>MKKLVMTAAVAAILGAASPVMAQGIPVFDGTRALDFVQQFARMKEQLDTAKDQLAEAQRMYEAVTGGRGLGDLMRNAQLREYLPDDLRTVYDSANGGGYSGISGSINDILRDERLNGSVADMRRSIEERSRTAAATDKAVGLRAYEGAQQRLAQIEGLMDEISRTQDQKAIEELQARIAGEQAAIQNETTKLQMIAQLRQAEQALISEQRRERNMRILSSGNQGMPTIQ[5x];>MSKKQPKPVKAEQLKSYYEESRGLERDLIGEFVKSRKTAWRVATASGLFGLLGMVCGIVGFSQPAPAPLVLRVDNATGAVDVVTTLREHESSYGEVVDTYWLNQYVLNREAYDYNTIQMNYDTTALLSAPAVQQDYYKLFDGSNARDRVLGNKARITVRVRSIQPNGRGQATVRFTTQQHNSNGTVEAPQHQIATIGYTYIGAPMRSSDRLLNPLGFQVTSYRADPEILNN[12x];>[5x]MAFELFTPLFNKIDQTTATYVTDISSRAIAAITPVVSVGLTLGFITYGWLIIRGAVEMPVAEFLNRCLRIGIIVSIALAGGLYQGEIANAITTVPDELASALLGNPTQGASAAALVDQSAQQGFDRASEAFEEAGFFSSDGLLYGLFGIIILLATGLLAAIGGAFLLLAKIALALLAGLGPLFILALIWQPTHRFFDQWAQQVLNYGLLIVLFAAVFGLLMQIFGSYMADLRFDGAQNVAYAIGGSVILSIVSIVLLMQLPSIASGLAGGIGLGYMWELRSMRSGAGAAMRGGRAMARGARAAPGAARGAAVGAANMAKTVATGGAGVARAAAGYFRGRKAG;>MGAIESRKLLASETPVGQFIPYSHHVTDTIISTKNAEYLSVWKIDGRSHQSASEADVFQWIRELNNTLRGISSANLSLWTHIVRRRVYEYPDAEFDNVFCRQLDEKYRESFTGYNLMVNDLYLTVVYRPVSDKVLSFFAKRERETPDQKKHRQESCIKALEDINRTLGQSFKRYGAELLSVYEKGGHAFSAPLEFLARLVNGEHIPMPICRDRFSDYMAVNRPMFSKWGEVGELRSLTGLRRFGMLEIREYDDATEPGQLNVLLESDYEFVLTHSFSVLSRPAAKEYLQRHQKNLIDARDVATDQIEEIDEALNQLISGHFVMGEHHCTLTVYGETVQQVRDNLAHASAAMLDVAVLPKPVDLALEAGYWAQLPANWQWRPRPAPITSLNFLSFSPFHNFMSGKPTGNPWGPAVTIL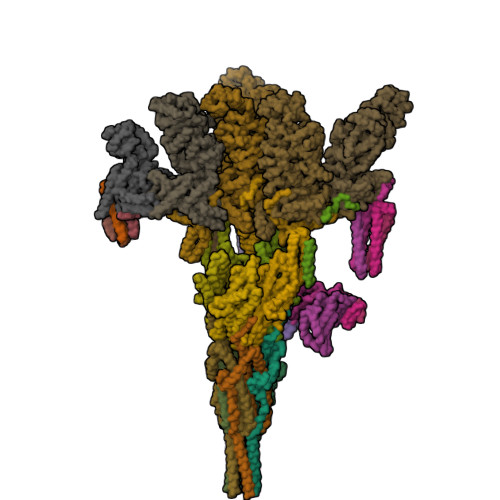KTVSGTPLYFNFHASKEEEDATDKRLLGNTMLIGQSSSGKTVLLGFLLAQAQKFKPTIVAFDKDRGMEISIRAMGGRYLPLKTGEPSGFNPFQLPPTHANLIFLKQFVKKLAAAGGEVTHRDEEEIDQAITAMMSDSIDKSLRRLSLLLQFLPNPRSDDMDARPTVHARLVKWCEGGDYGWLFDNPTDALDLSTHQIYGFDITEFLDNPEARTPVMMYLLYRTESMIDGRRFMYVFDEFWKPLQDEYFEDLAKNKQKTIRKQNGIFVFATQEPSDALESNIAKTLIQQCATYIFLANPKADYEDYTQGFKLTDSEFELVRGLGEFSRRFLIKQGDQSALAEMNLGKFRTIVDGETVERDFDDELLVLSGTPDNAEIAESIIAEVGDDPAVWLPIFLDRVKAERSDV[6x];>MKPPQQQHEAFPLFKGATRLPTIWGVPMIPLMAMVMGVAVIALTVSIWWWALVPPLWFIMAQITKNDDKAFRIWWLWIDTKFRNRNKGFWGASSYSPANYRKRR[3x];>[3x]MFGRKKGDVIDAGAELERAEQERIEGEYGASELASERRPHTPGARTLLMVLLCVIAVVLVTLSYKAYKVRGVVEDDDAQPQQVVRQVIPGYTPRPIRPEPENVPEPPQPTTSVPAIQPAPVTQPVRPQPTGPREKTPYELARERMLRSGLTAGSGGGEDLPRPQGGDVPAGGLMGGGGGGGELAEKLQPMRLSGSSAGRLGNRDMLITQGTQLDCVLETRLVTTQPGMTTCHLTRDVYSTSGRVVLLDRGSKVVGFYQGGLRQGQARIFVQWSRIETPSGVVINLDSPGTGPLGEAGLGGWIDRHFWERFGGAIMISLIGDLGDWASRQGSRQGDNSIQFSNTANGVESAAAEALRNSINIPPTLYKNQGERVNILVARDLDFSDVYSLESIPTK> MSIVTKSIVNADAEAR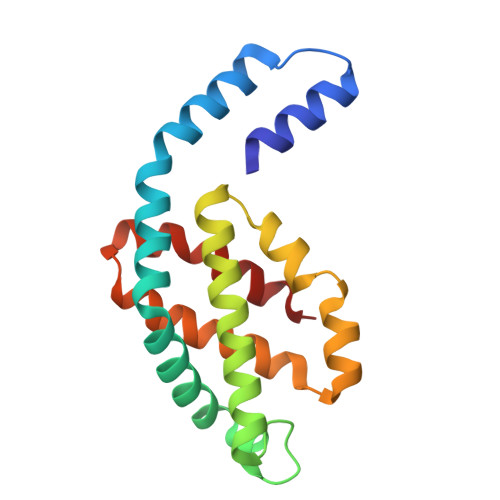YLSPGELDRIKGFVTSGERRLRIAQVLTESRERIVKQAGDQLFQKRPDVVSPGGNAYGEEMTATCLRDMDYYLRLITYGVVAGDVTPIEEIGLVGVREMYNSLGTPIPAVAEAVRCMKSVASSLLSGEDAAEAASYFDYVVGAMQ>[2x]MGHHHHHHSHMASSSVSISHSASATGNVCIEEIDVDGKFIRLKNTSEQDQPMGGWEMIRKIGDTSVSYKYTSRYVLKAGQTVTIWAANAGVTASPPTDLIWKNQNSWG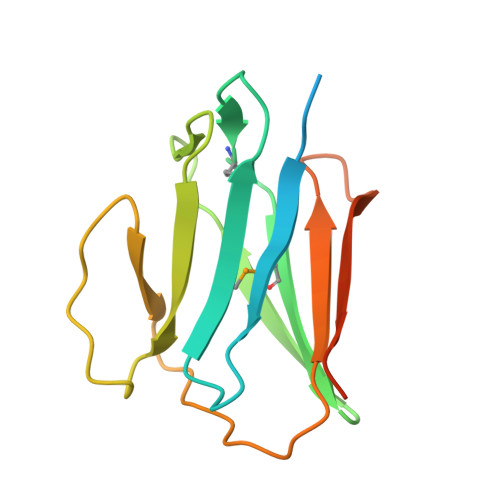TGEDVKVILKNSQGEEVAQRSTVFKTTIPEEEEEEE>[2x]PKKQTRLGLEAKKEENLADWYSQVITKSEMIEYHDISGCYILRPWAYAIWEAIKDFFDAEIKKLGVENCYFPMFVSQSALEKEKTHVADFAPEVAWVTRSGKTELAEPIAIRPTSETVMYPAYAKWVQSHRDLPIKLNQWCNVVRWEFKHPQPFLRTREFLWQEGHSAF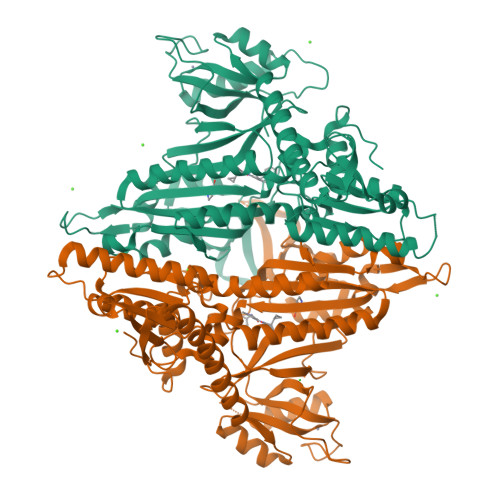ATMEEAAEEVLQILDLYAQVYEELLAIPVVKGRKTEKEKFAGGDYTTTIEAFISASGRAIQGGTSHHLGQNFSKMFEIVFEDPKIPGEKQFAYQNSWGLTTRTIGVMTMVHGDNMGLVLPPRVACVQVVIIPCGITNALSEEDKEALIAKCNDYRRRLLSVNIRVRADLRDNYSPGWKFNHWELKGVPIRLEVGPRDMKSCQFVAVRRDTGEKLTVAENEAETKLQAILEDIQVTLFTRASEDLKTHMVVANTMEDFQKILDSGKIVQIPFCGEIDCEDWIKKTTARDQDLEPGAPSMGAKSLCIPFKPLCELQPGAKCVCGKNPAKYYTLFGRSY>[2x]XIPAF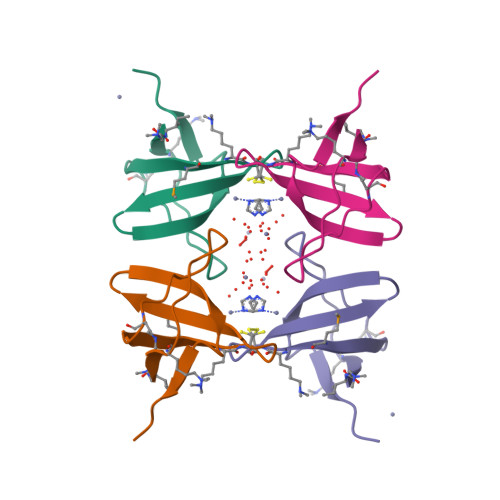VKFAYVAEREDELSLVKGSRVTVMEKCSDGWWRGSYNGQIGWFPSNYVLEEVD As the first reported host of “non-pathogenic-derived” pili, Lactobacillus rhamnosus GG is a gut-adapted commensal lactic acid bacterium (LAB) and one of many clinically investigated probiotic strains for human use in the prevention and treatment of certain gastric ailments. As with other Gram-positive bacteria, sortase-dependent piliation in L. rhamnosus GG (called SpaCBA) is assembled from the ~30 kDa SpaA (backbone), ~20 kDa SpaB (basal), and ~90 kDa SpaC (tip-located) pilins. Two immunoglobulin (Ig)-like subdomains comprise GG-SpaA, each having the conserved residues of a canonical E-box motif and internal isopeptide bonds formed between either lysine and asparagine or lysine and aspartate residues. Our findings show that the GG-SpaA structure has certain features in common with other pathogen-derived pilin-proteins, such as the Ig-like CnaB-type folds and the presence of internal isopeptide bonds6940.

Although the E139A mutant had been isolated using the same purification protocol used for WT protein, these conditions resulted in protein degradation when E269A-substituted GG-SpaA was purified. This was remedied by modifying the purification buffer. Here, this allowed for the recovery of intact and pure E269A mutant protein in both a monomeric (E2) and trimeric (E1) form, as evidenced by size-exclusion chromatographic analysis. Crystals of full-length E269A-substituted GG-SpaA had formed after three months for the E1 and E2 protein samples (for details), each having the same space groups and similar unit-cell edges as determined for the WT form. Moreover, the overall topological similarity of the E269A crystal structure to that of WT GG-SpaA, and including the molecular arrangement in the asymmetric unit, is high (RMSD of 0.4 Å). Surprisingly, electron density for an intact isopeptide bond is found between Lys184 and Asp295, despite the absence of the glutamate residue at position 269. Intriguingly, the alanine substitution of the C-terminal E-box glutamate (E269A) that presumably catalyzes K-D isopeptide bond formation had shown two contrasting structural effects. Here, this E-box mutation initially produced a crystal structure of the truncated N-domain lacking the K-N isopeptide bond (see further below), but then afterward, with the overall fold being retained where an intact K-D isopeptide bond was still visible in the C-domain. Up till now, this latter bonding behavior had never been observed, as in all known pilin structures, either a glutamate or an aspartate found in the vicinity of an isopeptide bond is directly associated with the bond-making process. Surprisingly, the mutation of E269 in the C-domain had no influence on K-N or K-D isopeptide formation.

>[3x]MGRDPNSTNDTTTQNVVLTKYGFDKDVTAIDRATDQIWTGDGAKPLQGVDFTIYNVTANYWASPKDYKGSFDSAPVAATGTTNDKGQLTQALPIQSKDASGKTRAAVYLFHETNPRAGYNTSADFWLTLPAKAAADGNVYVYPKNVQKTTYERTFVKKDAETKEVLEGAGFKISNSDGKFLKLTDKDGQSVSIGEGFIDVLANNYRLTWVAESDATVFTSDKSGKFGLNGFADNTTTYTAVATNVPDGYDAAANTDFKADNSSSDILDAPSGILPLEHHHHHH>MHHHHHHMLPKDFQWGFATAAYQIEGAVDQDGRGPSIWDTFCAQPGKIADGSSGVTACDSYNRTAEDIALLKSLGAKSYRFSISWSRIIPEGGRGDAVNQAGIDHYVKFVDDLLDAGITPFITLFHWDLPEGLHQRYGGLLNRTEFPLDFENYARVMFRALPKVRNWITFNEPLCSAIPGYGSGTFAPGRQSTSEPWTVGHNILVAHGRAVKAYRDDFKPASGDGQIGIVLNGDFTYPWDAADPADKEAAERRLEFFTAWFADPIYLGDYPASMRKQLGDRLPTFTPEERALVHGSNDFYGMNHYTSNYIRHRSSPASADDTVGNVDVLFTNKQGNCIGPETQSPWLRPCAAGFRDFLVWISKRYGYPPIYVTENGTSIKGESDLPKEKILEDDFRVKYYNEYIRAMVTAVELDGVNVKGYFAWSLMDNFEWADGYVTRFGVTYVDYENGQKRFPKKSAKSLKPLFDE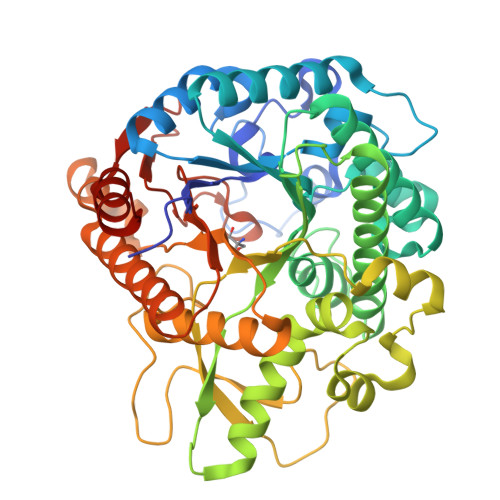LIAAA[4x]> MRTEDLPKAVVFLEPQWYSVLEKDSVTLKCQGAYSPEDNSTQWFHNESLISSQASSYFIDAATVNDSGEYRCQTNLSTLSDPVQLEVHIGWLLLQAPRWVFKEEDPIHLRCHSWKNTALHKVTYLQNGKDRKYFHHNSDFHIP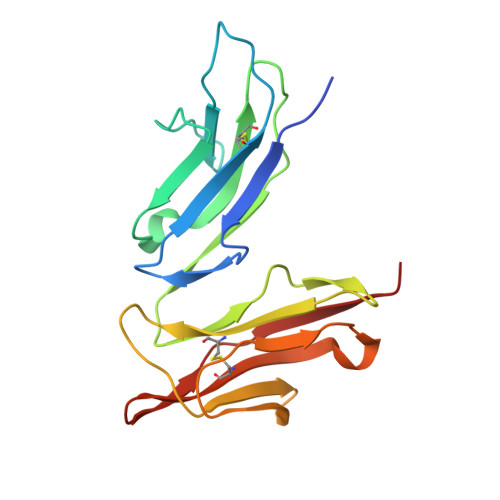KATLKDSGSYFCRGLVGSKNVSSETVNITITQG> UAAAA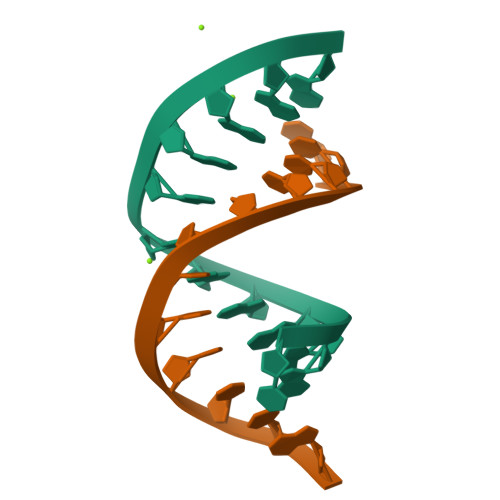GAAAAGG;> CCTTTTCTTTTA> MFIINSDFHRGNMEQYQKAQKLSFDPAELLRTSLNVGDIVLLKQCTSELTMCVNLPQSTTDPRYTFAKKDGTLVYAMKNSVILRIPKDLPEEVNQLLKRESNHPYQKIGTIKNSSNETEILPVLTRQLIVSFTLATFTKFAWTQLPIVLKKLELIHRYLQDSRGSKHVNFMSLVRIIKNLNIKEATDAINGDAYVRKVIDESMSVVNKSIDPTTLLATYWGVREQ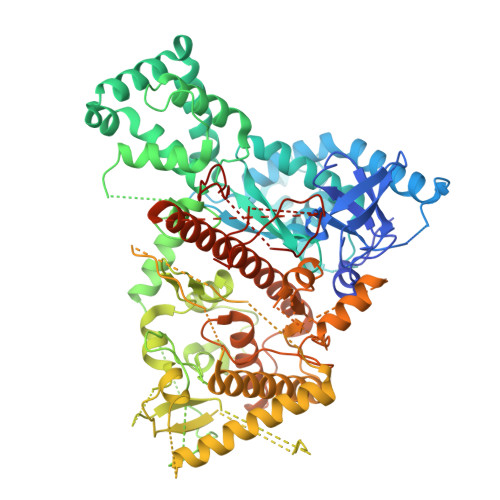QQNNLWGSVYTNTALLSPTTVAVLPLKKAHLFYQEVITRLESNDYQEIKAFAKLVNDKDYHSIAKRYDYIRTLLNDYAAGNIEENAVLTTIISKIFRHIDMYRDQDVTRSLCGKLLVEISPQSNSSNFILGNWDLNIPKSSGISSVEQKLYDTAMPTIVSDTDRYDFGDMPVFCIDSEDAHEINDGISIEELDGVRSRIHIHIADPAGLFPESFDYTKSGISDDVLRVSLKRAFTTYLPDLVVPMLPKSFCNRADLGKHDRKTETISFSFELVNKEDGGLHVDYDTFQVRLGIVSNFPKVTYDKVDSILNGDDNSLPSKQKKQLELLHTLATKLLHKRIHDDNAVVFGDGFNKGLVSLSPDDDGELCIPTFYDQSQTKSTLLVSEFMILTNKLCAAFFQENKIPGVYRCYNGLNLGNQAKAQFELLKENIKLGKLPSLKDITKISSQLSSSFYSPFPLPHKMIGNTAYLTVTSPMRRGPDLINHLQLHRFLKKLPLCFKQEYLDQYVWSFQARADILKIFQRHSSTYWTLKHLEQSGTKTHDVIVTSVPQNGTVNCLFPEYSYARGTLKLDPAMKKIPRIGDTIRHCKVESIHPLDGILTLTHVNRK>[2x]MARAAFLFKTVGFGGLQNVPINDELSSHLLRAGNSPWQLTQFLDWISLGRGLATSALVPTAGSRYYQMSCLLSGTLQIPFRPNHRWGDIRFLRLVWSAPTLDGLVVAPPQVLAQPALQAQADRVYDCDDYPFLARDPRFKHRVYQQLSAVTLLNLTGFGPISYVRVDEDMWSGDVNQLLMNYFGHTFAEIAYTLCQASANRPWEYDGTYARMTQIVLSLFWLSYVGVIHQQNTYRTFYFQCNRRGDAAEVWILSCSLNHSAQIRPGNRSLFVMPTSPDWNMDVNLILSSTLTGCLCSGSQLPLIDNNSVPAVSRNIHGWTGRAGNQLHGFQVRRMVTEFCDRLRRDGVMTQAQQNQVEALADQTQQFKRDKLETWAREDDQYNQAHPNSTMFRTKPFTNAQWGRGNTGATSAAIAALI;>[6x]MGNASSIVQTINVTGDGNVFKPSAETSSTAVPSLSLSPGMLNPGGVPWIAVGDETSVTSPGALRRMTSKDIPETAIINTDNSSGAVPSESALVPYIDEPLVVVTEHAITNFTKAEMALEFNREFLDKMRVLSVSPKYSDLLTYVDCYVGVSARQALNNFQKQVPVITPTRQTMYVDSIQAALKALEKWEIDLRVAQTLLPTNVPIGEVSCPMQSVVKLLDDQLPDDSLIRRYPKEAAVALAKRNGGIQWMDVSEGTVMNEAVNAVAASALAPSASAPPLEEKSKLTEQAMDLVTAAEPEIIASLAPVPAPVFAIPPKPADYNVRTLRIDEATWLRMIPKSMNTPFQIQVTDNTGTNWHLNLRGGTRVVNLDQIAPMRFVLDLGGKSYKETSWDPNGKKVGFIVFQSKIPFELWTAASQIGQATVVNYVQLYAEDSSFTAQSIIATTSLAYNYEPEQLNKTDPEMNYYLLATFIDSAAITPTNMTQPDVWDALLTMSPLSAGEVTVKGAVVSEVV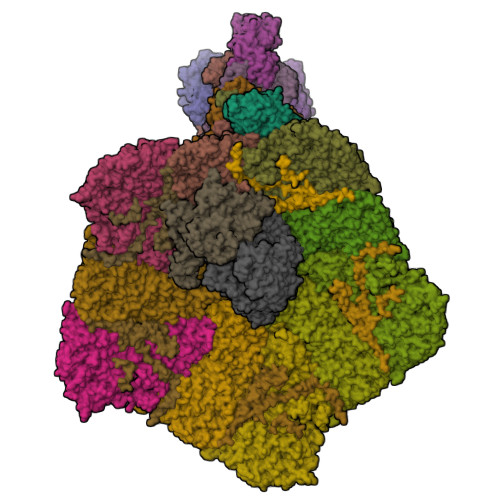PADLIGSYTPESLNASLPNDAARCMIDRASKIAEAIKIDDDAGPDEYSPNSVPIQGQLAISQLETGYGVRIFNPKGILSKIASRAMQAFIGDPSTIITQAAPVLSDKNNWIALAQGVKTSLRTKSLSAGVKTAVSKLSSSESIQNWTQGFLDKVSAHFPAPKPDCPTSGDSGESSNRRVKRDSYAGVVKRGYTR;>[3x]MEVCLPNGHQVVDLINNAFEGRVSIYSAQEGWDKTISAQPDMMVCGGAVVCMHCLGVVGSLQRKLKHLPHHRCNQQIRHQDYVDVQFADRVTAHWKRGMLSFVAQMHEMMNDVSPDDLDRVRTEGGSLVELNWLQVDPNSMFRSIHSSWTDPLQVVDDLDTKLDQYWTALNLMIDSSDLIPNFMMRDPSHAFNGVKLGGDARQTQFSRTFDSRSSLEWGVMVYDYSELEHDPSKGRAYRKELVTPARDFGHFGLSHYSRATTPILGKMPAVFSGMLTGNCKMYPFIKGTAKLKTVRKLVEAVNHAWGVEKIRYALGPGGMTGWYNRTMQQAPIVLTPAALTMFPDTIKFGDLNYPVMIGDPMILG;> MANVWGVRLADSLSSPTIETRTRQYTLHDLCSDLDANPGREPWKPLRNQRTNNIVAVQLFRPLQGLVLDTQLYGFPGAFDDWERFMREKLRVLKYEVLRIYPISNYSNEHVNVFVANALVGAFLSNQAFYDLLPLLIINDTMIGDLLGTGASLSQFFQSHGDVLEVAAGRKYLQMENYSNDDDDPPLFAKDLSDYAKAFYSDTYEVLDRFFWTHDSSAGVLVHYDKPTNGHHYLLGTLTQMVSAPPYIINATDAMLLESCLEQFSANVRARPAQPVTRLDQCYHLRWGAQYVGEDSLTYRLGVLSLLATNGYQLARPIPRQLTNRWLSSFVSQIMSDGVNETPLWPQERYVQIAYDSPSVVDGATQYGYVRKNQLRLGMRISALQSLSDTPSPVQWLPQYTIDQAAMDEGDLMVSRLTQLPLRPDYGNIWVGDALSYYVDYNRSHRVVLSSELPQLPDTYFDGDEQYGRSLFSLARKIGDRSLVKDTAVLKHAYQAIDPNTGKEYLRSRQSVAYFGASAGHSGADQPLVIEPWIQGKISGVPPPSSVRQFGYDVARGAIVDLARPFPSGDYQFVYSDVDQVVDGHDDLSISSGLVESLLSSCMHATAPGGSFVVKINFPTRPVWHYIEQKILPNITSYMLIKPFVTNNVELFFVAFGVHQHSSLTWTSGVYFFLVDHFYRYETLSTISRQLPSFGYVDDGSSVTGIETISIENPGFSNMTQAARIGISGLCANVGNARKSIAIYESHGARVLTITSRRSPASARRKSRLRYLPLIDPRSLEVQARTILPADPVLFENVSGASPHVCLTMMYNFEVSSAVYDGDVVLDLGTGPEAKILELIPATSPVTCVDIRPTAQPSGCWNVRTTFLELDYLSDGWITGVRGDIVTCMLSLGAAAAGKSMTFDAAFQQLIKVLSKSTANVVLVQVNCPTDVVRSIKGYLEIDSTNKRYRFPKFGRDEPYSDMDALEKICRTAWPNCSITWVPLSYDLRWTRLALLESTTLSSASIRIAELMYKYMPIMRIDIHGLPMEKRGNFIVGQNCSLVIPGFNAQDVFNCYFNSALAFSTEDVNAAMIPQVSAQFDATKGEWTLDMVFSDAGIYTMQALVGSNANPVSLGSFVVDSPDVDITDAWPAQLDFTIAGTDVDITVNPYYRLMTFVRIDGQWQIANPDKFQFFSSASGTLVMNVKLDIADKYLLYYIRDVQSRDVGFYIQHPLQLLNTITLPTNEDLFLSAPDMREWAVKESGNTICILNSQGFVLPQDWDVLTDTISWSPSIPTYIVPPGDYTLTPL;>MKRIPRKTKGKSSGKGNDSTERADDGSSQLRDKQNNKAGPATTEPGTSNREQYKARPGIASVQRATESAEMPMKNNDEGTPDKKGNTKGDLVNEHSEAKDEADEATKKQAKDTDKSKAQVTYSDTGINNANELSRSGNVDNEGGSNQKPMSTRIAEATSAIVSKHPARVGLPPTASSGHGYQCHVCSAVLFSPLDLDAHVASHGLHGNMTLTSSDIQRHITEFISSWQNHPIVQVSADVENKKTAQLLHADTPRLVTWDAGLCTSFKIVPIVPAQVPQDVLAYTFFTSSYAIQSPFPEAAVSRIVVHTRWASNVDFDRDSSVIMAPPTENNIHLFKQLLNTETLSVRGANPLMFRANVLHMLLEFVLDNLYLNRHTGFSQDHTPFTEGANLRSLPGPDAEKWYSIMYPTRMGTPNVSKICNFVASCVRNRVGRFDRAQMMNGAMSEWVDVFETSDALTVSIRGRWMARLARMNINPTEIEWALTECAQGYVTVTSPYAPSVNRLMPYRISNAERQISQIIRIMNIGNNATVIQPVLQDISVLLQRISPLQIDPTIISNTMSTVSESTTQTLSPASSILGKLRPSNSDFSSFRVALAGWLYNGVVTTVIDDSSYPKDGGSVTSLENLWDFFILALALPLTTDPCAPVKAFMTLANMMVGFETIPMDNQIYTQSRRASAFSTPHTWPRCFMNIQLISPIDAPILRQWAEIIHRYWPNPSQIRYGAPNVFGSANLFTPPEVLLLPIDHQPANVTTPTLDFTNELTNWRARVCELMKNLVDNQRYQPGWTQSLVSSMRGTLDKLKLIKSMTPMYLQQLAPVELAVIAPMLPFPPFQVPYVRLDRDRVPTMVGVTRQSRDTITQPALSLSTTNTTVGVPLALDARAITVALLSGKYPPDLVTNVWYADAIYPMYADTEVFSNLQRDMITCEAVQTLVTLVAQISETQYPVDRYLDWIPSLRASAATAATFAEWVNTSMKTAFDLSDMLLEPLLSGDPRMTQLAIQYQQYNGRTFNIIPEMPGSVIADCVQLTAEVFNHEYNLFGIARGDIIIGRVQSTHLWSPLAPPPDLVFDRDTPGVHIFGRDCRISFGMNGAAPMIRDETGLMVPFEGNWIFPLALWQMNTRYFNQQFDAWIKTGELRIRIEMGAYPYMLHYYDPRQYANAWNLTSAWLEEITPTSIPSVPFMVPISSDHDISSAPAVQYIISTEYNDRSLFCTNSSSPQTIAGPDKHIPVERYNILTNPDAPPTQIQLPEVVDLYNVVTRYAYETPPITAVVMGVP[15x];> MAYIAVPAVVDSRSSEAIGLLESFGVDAGADANDVSYQDHDYVLDQLQYMLDGYEAGDVIDALVHKNWLHHSVYCLLPPKSQLLEYWKSNPSAIPDNVDRRLRKRLMLKKDLRKDDEYNQLARAFKISDVYAPLISSTTSPMTMIQNLNQGEIVYTTTDRVIGARILLYAPRKYYASTLSFTMTKCIIPFGKEVGRVPHSRFNVGTFPSIATPKCFVMSGVDIESIPNEFIKLFYQRVKSVHANILNDISPQIVSDMINRKRLRVHTPSDRRAAQLMHLPYHVKRGASHVDVYKVDVVDMLFEVVDVADGLRNVSRKLTMHTVPVCILEMLGIEIADYCIRQEDGMLTDWFLLLTMLSDGLTDRRTHCQYLINPSSVPPDVILNISITGFINRHTIDVMPDIYDFVKPIGAVLPKGSFKSTIMRVLDSISILGIQIMPRAHVVDSDEVGEQMEPTFEQAVMEIYKGIAGVDSLDDLIKWVLNSDLIPHDDRLGQLFQAFLPLAKDLLAPMARKFYDNSMSEGRLLTFAHADSELLNANYFGHLLRLKIPYITEVNLMIRKNREGGELFQLVLSYLYKMYATSAQPKWFGSLLRLLICPWLHMEKLIGEADPASTSAEIGWHIPREQLMQDGWCGCEDGFIPYVSIRAPRLVIEELMEKNWGQYHAQVIVTDQLVVGEPRRVSAKAVIKGNHLPVKLVSRFACFTLTAKYEMRLSCGHSTGRGAAYSARLAFRSDLA;> MSSMILTQFGPFIESISGITDQSNDVFEDAAKAFSMFTRSDVYKALDEIPFSDDAMLPIPPTIYTKPSHDSYYYIDALNRVRRKTYQGPDDVYVPNCSIVELLEPHETLTSYGRLSEAIENRAKDGDSQARIATTYGRIAESQARQIKAPLEKFVLALLVAEAGGSLYDPVLQKYDEIPDLSHNCPLWCFREICRHISGPLPDRAPYLYLSAGVFWLMSPRMTSAIPPLLSDLVNLAILQQTAGLDPSLVKLGVQICLHAAASSSYAWFILKTKSIFPQNTLHSMYESLEGGYCPNLEWLEPRSDYKFMYMGVMPLSAKYARSAPSNDKKARELGEKYGLSSVVGELRKRTKTYVKHDFASVRYIRDAMACTSGIFLVRTPTETVLQEYTQSPEIKVPIPQKDWTGPIGEIRILKDTTSSIARYLYRTWYLAAARMAAQPRTWDPLFQAIMRSQYVTARGGSGAALRESLYAINVSLPDFKGLPVKAATKIFQAAQLANLPFSHTSVAILADTSMGLRNQVQRRPRSIMPLNVPQQQVSAPHTLTADYINYHMNLSTTSGSAVIEKVIPLGVYASSPPNQSINIDISACDASITWDFFLSVIMAAIHEGVASSSIGKPFMGVPASIVNDESVVGVRAARPISGMQNMIQHLSKLYKRGFSYRVNDSFSPGNDFTHMTTTFPSGSTATSTEHTANNSTMMETFLTVWGPEHTDDPDVLRLMKSLTIQRNYVCQGDDGLMIIDGTTAGKVNSETIQKMLELISKYGEEFGWKYDIAYDGTAEYLKLYFIFGCRIPNLSRHPIVGKERANSSAEEPWPAILDQIMGVFFNGVHDGLQWQRWIRYSWALCCAFSRQRTMIGESVGYLQYPMWSFVYWGLPLVKAFGSDPWIFSWYMPTGDLGMYSWISLIRPLMTRWMVANGYVTDRCSPVFGNADYRRCFNELKLYQGYYMAQLPRNPKKSGRAAPREVREQFTQALSDYLMQNPELKSRVLRGRSEWEKYGAGIIHNPPSLFDVPHKWYQGAQEAAIATREELAEMDETLMRARRHSYSSFSKLLEAYLLVKWRMCEAREPSVDLRLPLCAGIDPLNSDPFLKMVSVGPMLQSTRKYFAQTLFMAKTVSGLDVNAIDSALLRLRTLGADKKALTAQLLMVGLQESEADALAGKIMLQDVNTVQLARVVNLAVPDTWMSLDFDSMFKHHVKLLPKDGRHLNTDIPPRMGWLRAILRFLGAGMVMTATGVAVDIYLEDIHGGGRSLGQRFMTWMRQEGRSA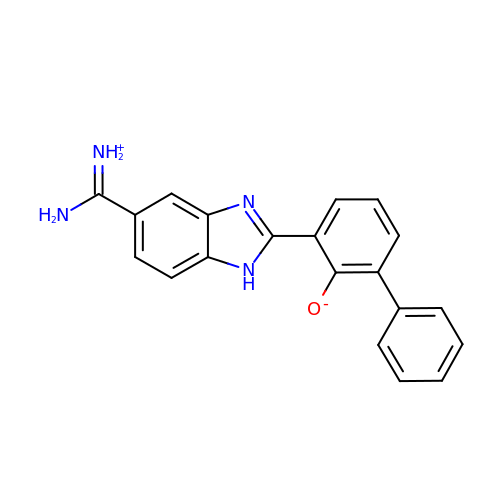3-{5-[AMINO(IMINIO)METHYL]-1H-BENZIMIDAZOL-2-YL}-1,1'-BIPHENYL-2-OLATE | C20 H16 N4 O | LMGQGPVCSYOMNS-UHFFFAOYSA-N>[2x]MASISRFRGCLAGALLGDCVGAVYEAHDTVSLASVLSHVESLEPDPGTPGSARTETLYYTDDTAMTRALVQSLLAKEAFDEVDMAHRFAQEYKKDPDRGYGAGVITVFKKLLNPKCRDVYEPARAQFNGKGSYGNGGAMRVAGISLAYSSVQDVQKFARLSAQLTHASSLGYNGAILQALAVHLALQGVSSSEHFLEQLLGHMEELEGDAQSVLDAKELGMEERPYSSRL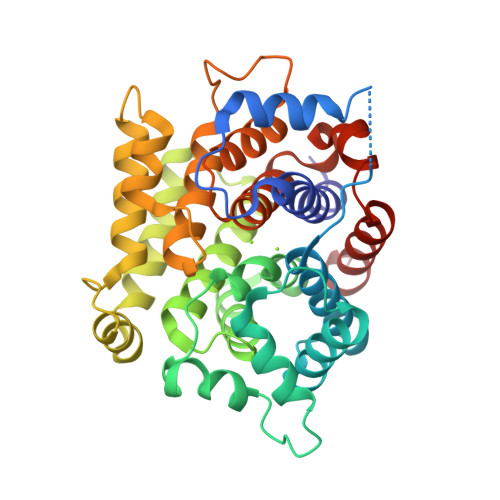KKVGELLDQDVVSREEVVSELGNGIAAFESVPTAIYCFLRCMEPHPEIPSTFNSLQRTLIYSISLGGDTDTIATMAGAIAGAYYGMEQVPESWQQSCEGFEETDVLAQSLHRVFQES> MAAIGRGRSLKNLRVRGRNDSGEENVPLDLTREPSDNLREILQNVARLQGVSNMRKLGHLNNFTKLLCDIGHSEEKLGFHYEDIIICLRLALLNEAKEVRAAGLRALRYLIQDSSILQKVLKLKVDYLIARCIDIQQSNEVERTQALRLVRKMITVNASLFPSSVTNSLIAVGNDGLQERDRMVRACIAIICELALQNPEVVALRGGLNTILKNVIDCQLSRINEALITTILHLLNHPKTRQYVRADVELERILAPYTDFHYRHSPDTAEGQLKEDREARFLASKMGIIATFRSWAGIINLCKPGNSGIQSLIGVLCIPNMEIRRGLLEVLYDIFRLPLPVVTEEFIEALLSVDPGRFQDSWRLSDGFVAAEAKTILPHRARSRPDLMDNYLALILSAFIRNGLLEGLVEVITNSDDHISVRATILLGELLHMANTILPHSHSHHLHCLPTLMNMAASFDIPKEKRLRASAALNCLKRFHEMKKRGPKPYSLHLDHIIQKAIATHQKRDQYLRVQKDIFILKDTEEALLINLRDSQVLQHKENLEWNWNLIGTILKWPNVNLRNYKDEQLHRFVRRLLYFYKPSSKLYANLDLDFAKAKQLTVVGCQFTEFLLESEEDGQGYLEDLVKDIVQWLNASSGMKPERSLQNNGLLTTLSQHYFLFIGTLSCHPHGVKMLEKCSVFQCLLNLCSLKNQDHLLKLTVSSLDYSRDGLARVILSKILTAATDACRLYATKHLRVLLRANVEFFNNWGIELLVTQLHDKNKTISSEALDILDEACEDKANLHALIQMKPALSHLGDKGLLLLLRFLSIPKGFSYLNERGYVAKQLEKWHREYNSKYVDLIEEQLNEALTTYRKPVDGDNYVRRSNQRLQRPHVYLPIHLYGQLVHHKTGCHLLEVQNIITELCRNVRTPDLDKWEEIKKLKASLWALGNIGSSNWGLNLLQEENVIPDILKLAKQCEVLSIRGTCVYVLGLIAKTKQGCDILKCHNWDAVRHSRKHLWPVVPDDVEQLCNELSSIPSTLSLNSESTSSRHNSESESVPSSMFILEDDRFGSSSTSTFFLDINEDTEPTFYDRSGPIKDKNSFPFFASSKLVKNRILNSLTLPNKKHRSSSDPKGGKLSSESKTSNRRIRTLTEPSVDFNHSDDFTPISTVQKTLQLETSFMGNKHIEDTGSTPSIGENDLKFTKNFGTENHRENTSRERLVVESSTSSHMKIRSQSFNTDTTTSGISSMSSSPSRETVGVDATTMDTDCGSMSTVVSTKTIKTSHYLTPQSNHLSLSKSNSVSLVPPGSSHTLPRRAQSLKAPSIATIKSLADCNFSYTSSRDAFGYATLKRLQQQRMHPSLSHSEALASPAKDVLFTDTITMKANSFESRLTPSRFMKALSYASLDKEDLLSPINQNTLQRSSSVRSMVSSATYGGSDDYIGLALPVDINDIFQVKDIPYFQTKNIPPHDDRGARAFAHDAGGLPSGTGGLVKNSFHLLRQQMSLTEIMNSIHSDASLFL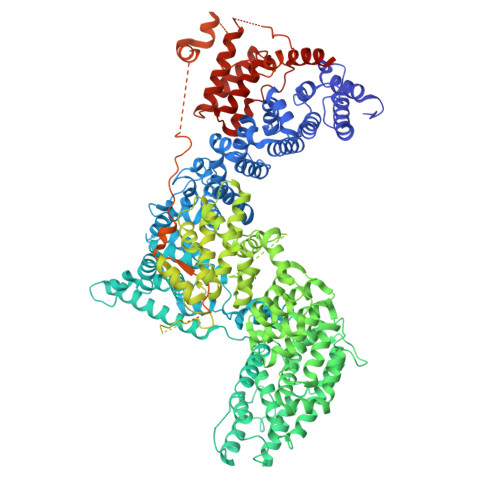ESTEDTGLQEHTDDNCLYCVCIEILGFQPSNQLSAICSHSDFQDIPYSDWCEQTIHNPLEVVPSKFSGISGCSDGVSQEGSASSTKSTELLLGVKTIPDDTPMCRILLRKEVLRLVINLSSSVSTKCHETGLLTIKEKYPQTFDDICLYSEVSHLLSHCTFRLPCRRFIQELFQDVQFLQMHEEAEAVLATPPKQPIVDTSAES>MVGLEDDTERERSPVVENGFSNGSRSSSSSAGVLSPSRKVTQGNDTLSYANILRARNKFADALALYEAMLEKDSKNVEAHIGKGICLQTQNKGNLAFDCFSEAIRLDPHNACALTHCGILHKEEGRLVEAAESYQKALMADASYKPAAECLAIVLTDLGTSLKLAGNTQEGIQKYYEALKIDPHYAPAYYNLGVVYSEMMQYDNALSCYEKAALERPMYAEAYCNMGVIYKNRGDLEMAITCYERCLAVSPNFEIAKNNMAIALTDLGTKVKLEGDVTQGVAYYKKALYYNWHYADAMYNLGVAYGEMLKFDMAIVFYELAFHFNPHCAEACNNLGVLYKDRDNLDKAVECYQMALSIKPNFAQSLNNLGVVYTVQGKMDAAASMIEKAILANPTYAEAFNNLGVLYRDAGNITMAIDAYEECLKIDPDSRNAGQNRLLAMNYINEGLDDKLFEAHRDWGWRFTRLHPQYTSWDNLKDPERPITIGYISPDFFTHSVSYFIEAPLTHHDYTKYKVVVYSAVVKADAKTYRFRDKVLKKGGVWKDIYGIDEKKIASMVREDKIDILVELTGHTANNKLGTMACRPAPVQVTWIGYPNTTGLPTVDYRITDSLADPPDTKQKQVEEL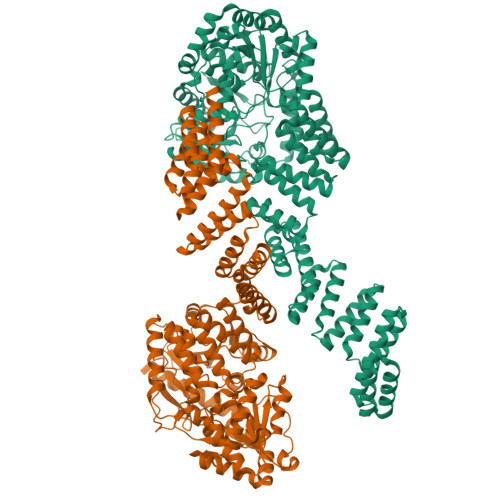VRLPDCFLCYTPSPEAGPVCPTPALSNGFVTFGSFNNLAKITPKVLQVWARILCAVPNSRLVVKCKPFCCDSIRQRFLTTLEQLGLESKRVDLLPLILFNHDHMQAYSLMDISLDTFPYAGTTTTCESLYMGVPCVTMAGSVHAHNVGVSLLTKVGLGHLVAKNEDEYVQLSVDLASDVTALSKLRMSLRDLMAGSPVCNGPSFAVGLESAYRNMWKKYCKGEVPSLRRMEMLQKEVHDDPLISKDLGPSRVSVTGEATPSLKANGSAPVPSSLPTQSPQLSKRMDSTSGGSENLYFQGGSHHHHHHHHHHGGWSHPQFEK[2x]>[2x]SMEGVIESNWNEIVDSFDDMNLSESLLRGIYAYGFEKPSAIQQRAILPCIKGYDVIAQAQSGTGKTATFAISILQQIELDLKATQALVLAPTRELAQQIQKVVMALGDYMGASCHACIGGTNVRAEVQKLQMEAPHIIVGTPGRVFDMLNRRYLSPKYIKMFVLDEADEMLSRGFKDQIYDIFQKLNSNTQVVLLSATMPSDVLEVTKKFMRDPIRILVKK

DExD/H-box RNA helicases, from virus and bacteria to eukaryotes, play important roles in processes including ribosome biogenesis, RNA processing and folding, ribonucleoprotein (RNP) remodeling, RNA nuclear export, the regulation of RNA translation and transcription, and nonsense-mediated RNA decay. DExD/H-box proteins often contain accessory regulatory domains and localization modules, but their cores consist of two RecA-like domains joined by a short flexible linker. The N-terminal domain is commonly referred to as conserved domain-1, or DEAD-domain, and the C-terminal domain as conserved domain-2, or helicase domain. Both domains contribute to the binding site for RNA substrates and both contribute to ATP hydrolysis. We used X-ray crystallography to determine the structures of the DEAD-domains of DDX2A, DDX2B, DDX5, DDX10, DDX18, DDX20, DDX47, DDX52, and DDX53, as well as the helicase domains of DDX25 and DDX41.

DDX2A (eIF4A1) is essential for translation initiation. It is part of the eIF4F complex that consists of eIF4G, eIF4E and eIF4A. The eIF4F complex and eIF4A are potential targets for anti cancer drugs. Motifs Ia, Ib and II seem unaffected by the state of ATP hydrolysis, and their conformations remain unchanged even in the crystal structures in which the nucleotide binding site is not occupied. In all single DEAD-domain structures, α-helix 8 has adopted a position that would block the RNA binding site.> VVKQDLSDNQYIQKKPNEITSNELLLPLPNDKLLGDPKAPILMIEYASLTCYHCSLFHRNVFPKIKEKYIDTGKMLYIFRHFPLDYRGLK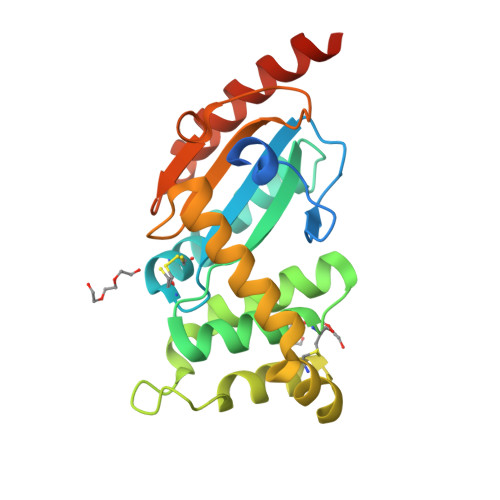AAMLSHCYEKQEDYFNFNKAVFNSIDSWNYYNLSDLTLLQRIAALSNLKQDAFNQCINDKKIMDKIVNDKSLAINKLGITATPIFFIKLNDDKSYIEHNKVKHGGYKELKYFTNVIDKLYGKAIVKLEHHHHHHHH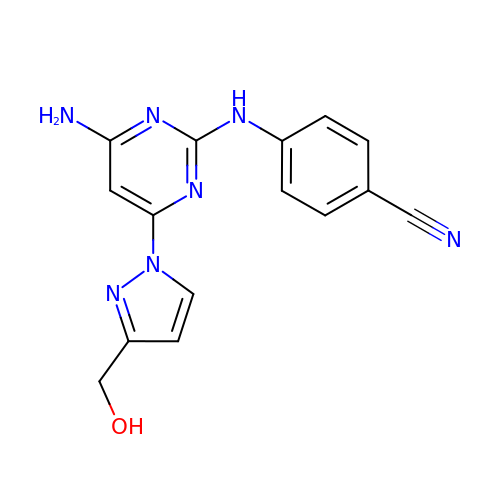4-({4-amino-6-[3-(hydroxymethyl)-1H-pyrazol-1-yl]pyrimidin-2-yl}amino)benzonitrile | C15 H13 N7 O | NMBKNACBCUDEER-UHFFFAOYSA-N>RSMAEEVSTLMKATVLMRQPGRVQEIVGALRKGGGDRLQVISDFDMT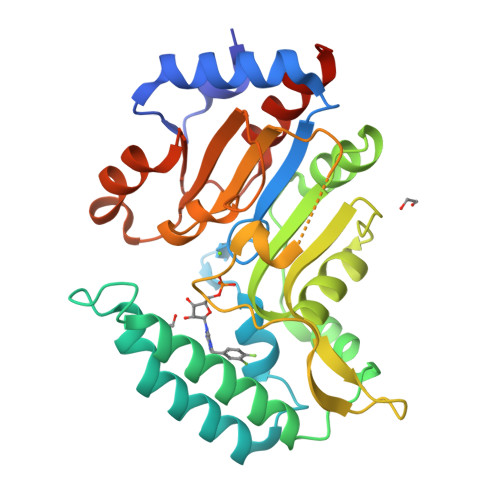LSRFAYNGKRCPSSYNILDNSKIISEECRKELTALLHHYYPIEIDPHRTVKEKLPHMVEWWTKAHNLLCQQKIQKFQIAQVVRESNAMLREGYKTFFNTLYHNNIPLFIFSAGIGDILEEIIRQMKVFHPNIHIVSNYMDFNEDGFLQGFKGQLIHTYNKNSSACENSGYFQQLEGKTNVILLGDSIGDLTMADGVPGVQNILKIGFLNDKVEERRERYMDSYDIVLEKDETLDVVNGLLQHILCQGVQLEMQGP[2x]> MITELRTKGATRTPAIRYSYPAPPPSKNAAPQQPRGTPRPRTAKTNVRKPKRSDARRRARAGSGFGVVSPVRARRRRVVGPPFADFFGALFPATRGIAFLSDLPTHIFSSFLLSFLAGRGVAMLRMC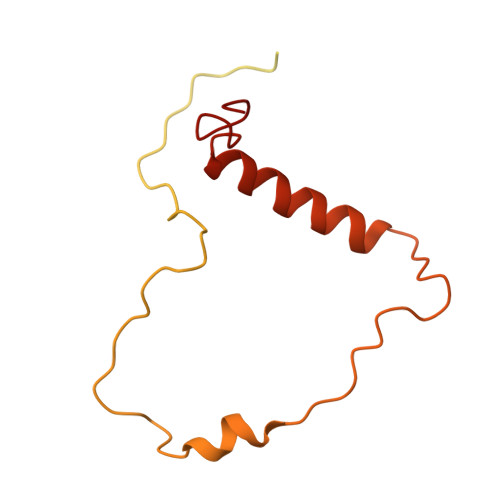RRLAMKYADLELTTRGEFPHGMKEPGFVKKLDQNIPWYFSTYRSMYHWPITGDNWSDLNEAEKHHDLHMFYTLAWWKLGEGIFDANDEDN>[2x]AAAAAAAAAA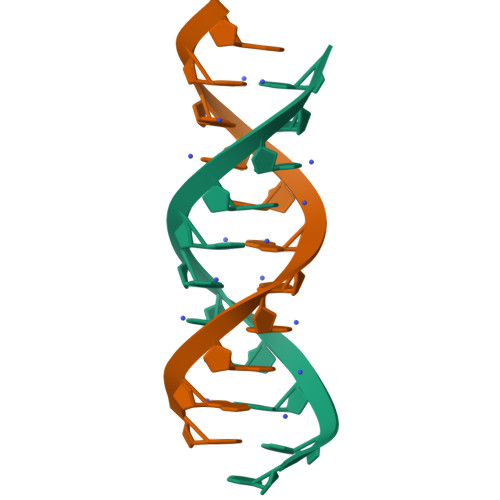A> MGSSHHHHHHLVPRGSPEAPYASLTEIEHLVQSVCKSYRETCQLRLEDLLRQRSNIFSREEVTGYQRKSMWEMWERCAHHLTEAIQYVVEFAKRLSGFMELCQNDQIVLLKAGAMEVVLVRMCRAYNADNRTVFFEGKYGGMELFRALGCSELISSIFDFSHSLSALHFSEDEIALYTALVLINAHRPGLQEKRKVEQLQYNLELAFHHHLCKTHRQSILAKLPPKGKLRSLCSQHVERLQIFQHLHP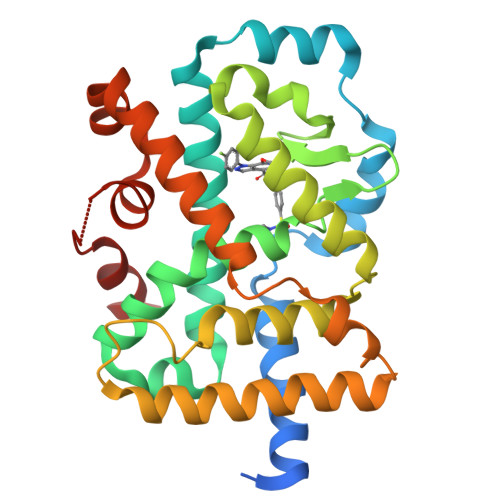IVVQAAFPPLYKELFSGGGEKHKILHRLLQDS> PKHGKRYRALLEKVDPNKIYTIDEAAHLVKELATAKFDETVEVHAKLGIDPRRSDQNVRGTVSLPHGLGKQVRVLAIAKGEKIKEAEEAGADYVGGEEIIQKILDGWMDFDAVVATPDVMGAVGSKMGRILGPRGLLPNPKAGTVGFNIGEIIREIKAGRIEFRNDKTGAIHAPVGKASFPP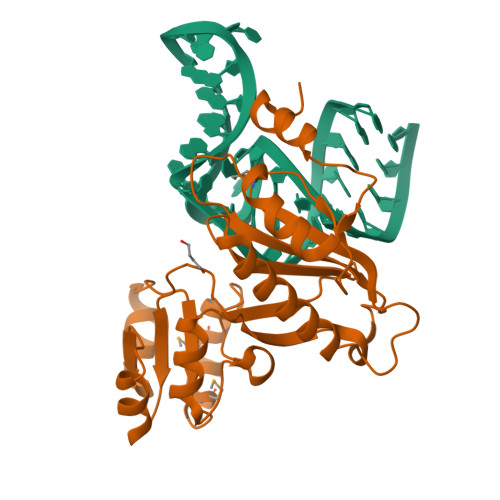EKLADNIRAFIRALEAHKPEGAKGTFLRSVYVTTTMGPSVRINPHS BETA-1,2,3,4,6-PENTA-O-GALLOYL-D-GLUCOPYRANOSE | C41 H32 O26 | 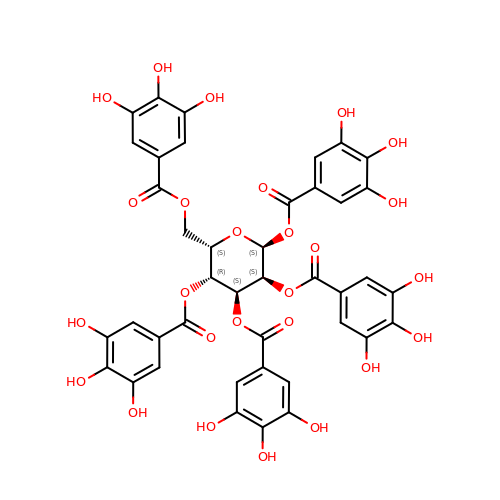QJYNZEYHSMRWBK-CGKDMBANSA-N>MTDLKASSLRALKLMDLSTLNGDYTDEKVIALCHQAKTPVGNTAAISIYPRSIPIARKTLKEQGTPEIRIATVTNFPHGNDDIEIALAETRAAIAYGADEVDVVFPYRALMAGNEQVGFDLVKACKEACAAANVLLKVIIESGELKDEALIRKASEISI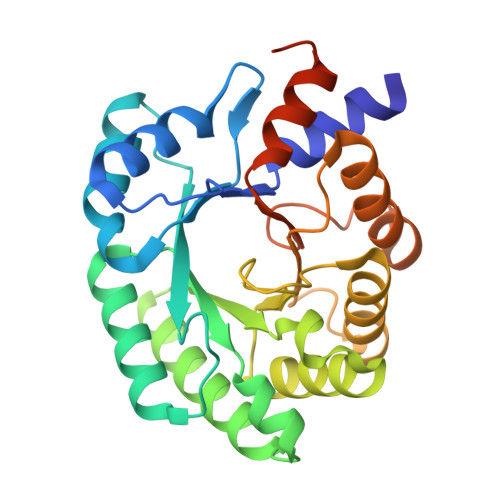KAGADFIKTSTGLVAVNATPESARIMMEVIRDMGVEKSVGFKVTGGARTAEDAQKYLAIADELFGADWADARHYRFGASGLLASLLKALGHGDGKSASSYLEHHHHHH[2x]> PHTNET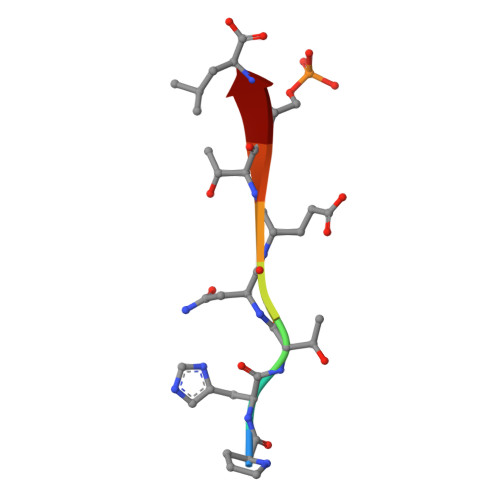SL>ALRETVVEVPQVTWEDIGGLEDV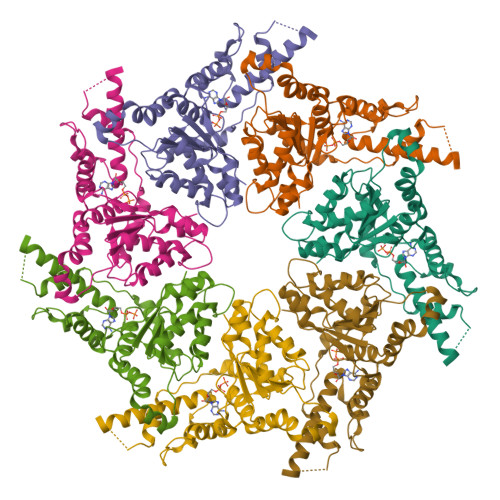KRELQELVQYPVEHPDKFLKFGMTPSKGVLFYGPPGCGKTLLAKAIANECQANFISIKGPELLTMWFGESEANVREIFDKARQAAPCVLFFDELDSIAKARGGNIGDGGGAADRVINQILTEMDGMSTKKNVFIIGATNRPDIIDPAILRPGRLDQLIYIPLPDEKSRVAILKANLRKSPVAKDVDLEFLAKMTNGFSGADLTEICQRACKLAIRESIESEIRRERERQTNPSAMEVEEDDPVPEIRRDHFEEAMRFARRSVSDNDIRKYEMFAQTLQ[14x]>MGVPAFFRWLTKKYPATVVNANEDRQRDQDGNRVPVDCTQPNPNFQEFDNLYLDMNGIIHPCTHPEDRPAPKNEDEMFALIFEYIDRIYSIVRPRRLLYMAIDGVAPRAKMNQQRSRRFRASKEMAEKEASIEEQRNRLMAEGIAVPPKKKEEAHFDSNCITPGTPFMARLADALRYYIHDRVTNDASWANIEIILSDANVPGEGEHKIMDYVRKQRGNPAHDPNTVHCLCGADADLIMLGIATHEANFNIIREEFVQREKNFIFLRIPVLREYLEKELSMPNLPFKFDVERALDDWVFLCFFVGNDFLPHLPSLEIREGAIDRLIKLYKEMVYQMKGYLTKDGIPELDRVEMIMKGLGRVEDEIFKRRQQDEERFQENQKDDIRLYESGWKDRYYRAKFDVGSDDIEFRHRVAWAYVEGLCWVLRYYYQGC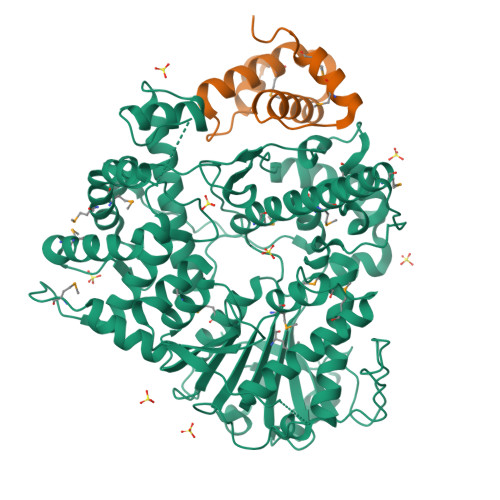ASWDWYFPYHYAPFASDFETVGEFQPDFTRPTKPFNPLEQLMSVFPAASKQHLPVEWQKLMIQDDSPIIDLYPADFRIDLNGKKYAWQGVALLPFVDETRLLATLQSVYPTLTAEEKQRNTRGPNRIFIGRNHKSFEFFQQVAESKSDDLVPLDPTLLNGVSGKIAYDSTATAPGLPFVSPVNHDECQDLPTNCGICVLYEDPE[6x];>GGGRGKLEDVEAEKKLWESDDAWELRKAFMLAHYDDYPKIQLQCLSQLFINVTLLGCEYSQTLMQKIRTMGAGIAANK[6x]> MKTAAIFALLAGSAAAFAPTTVSPRASTVAHMSSINEAFGISIETGNKCPPLGARILEDAQPSAIKWFQNAEIKHGRIAMVATI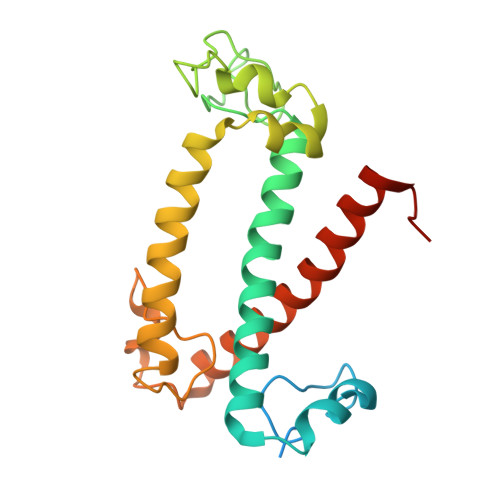GYLVQKLGVHFPLYLGPSGSNCFHPESETAWLLSSSTGVTFSDIAKAAPLDAIQMVPVAGWMQIFFVAGWFESVAYYRQWVKNSPIPGDYGYDPLGFTKREGGWDSEELTSLRLKEIKNGRLAMMTIAAWVSDEMIPGALPVWHP>SKTVSTINSTDALAMVEHSSELTLSITTPVGTKFVCRTPFIGTHTDKFLLVEMPKISADDLQYFFQEGFWMNIRAISPRGEGALIHFRSQLMHILQEPVPMAFLSIPNTMQVSQRRKEPRFELNLAGKVLFDEHRGDCELRDLS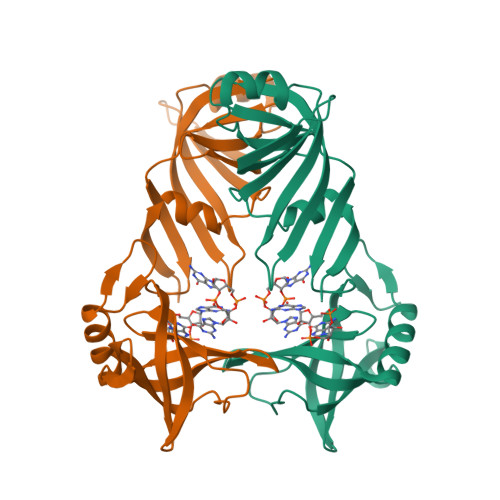RSGCRFITPPLGKTYQVGDLVALEIFSDLRGTKTFPPLTGKICNLQRSLHHARYGLEFNEEGRNNAKNLLAQLKFNGTKLTLN[2x]>MSKVISTPDAPAAIGPYCQARLCDRTLYTSGIIGNDPHGGPNPETVEGQAELIMKSLDAMLKAAGYEKTDVVKCNCYLADIADFQKFNKIYADYFGDHKPCRCCIQAGKLPAGKLVELDAIAYK[4x]

A perchloric-acid-soluble protein (PSP) named Tv-PSP1 was previously reported in T. vaginalis. We previously reported a perchloric-acid-soluble protein (PSP) from T. vaginalis named Tv-PSP1; this protein has a trimeric structure and may possess a putative ribonuclease function, although additional evidence suggests conflicting results due to the purification process with derivatization with chlorine. The L-PSP protein family possesses different biological functions and possible activity as a ribonuclease. The Tv-PSP1 protein from T. vaginalis is capable of binding stem-loop structures from RNAm.

We found the recombinant Tv-PSP1 structure, determined with X-ray crystallography, showed unusual thermal stability of the quaternary structure, associated with a disulfide bridge CYS76-CYS104. Each monomer of the asymmetric unit is part of one trimer formed by the same monomers from different asymmetric units. With respect to monomer folding, Tv-PSP1 maintains an antiparallel/parallel mixed beta sheet in order 123645, with two alpha helixes on one side, and the trimers form with closely packed beta sheets. We determined all structures through crystallographic studies: two of them (Tv-PSP1 A and B) have a single disulfide bond (CYS76-CYS104) with different B factors; another two (Tv-PSP1 C and D) have no evidence of any disulfide bond; and the last structure (Tv-PSP1 D) has a partial subunit due to its high vibrational motion state. Monomers C and D, with broken disulfide bridges, have high thermal stability (high average B factors) with respect to monomers A and B, which each contain a partial disulfide bridge. In the disulfide bridge, we observed a differential occupancy between A and B monomers with a tendency toward the A (75%) conformation, although the functional meaning of this is unclear. In other L-PSP1 proteins, the central area of the trimers contains a reduced cavity. These data suggest that the disulfide bridge does not function to maintain the trimer/fold protein, so may be a functional characteristic of Tv-PSP1. The structures show a potential second disulfide bridge between CYS18 and CYS101 from different monomers of the same trimer, which did not formed but are in close contact; this requires further studies to determine.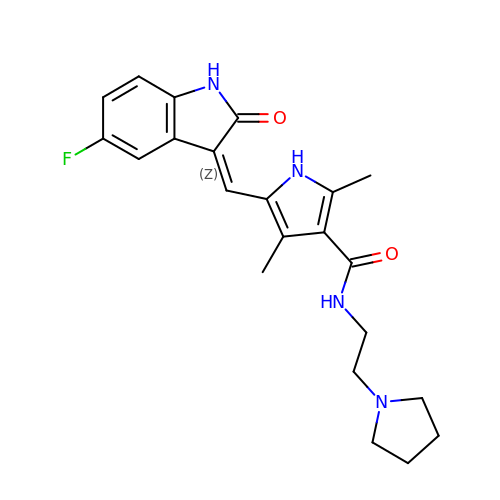5-[(Z)-(5-fluoranyl-2-oxidanylidene-1H-indol-3-ylidene)methyl]-2,4-dimethyl-N-(2-pyrrolidin-1-ylethyl)-1H-pyrrole-3-carboxamide | C22 H25 F N4 O2 | SRSGVKWWVXWSJT-ATVHPVEESA-N> GAMAQQKLDVKWIDKGINWIVYSAKDRENFTMDRWAKFYVNGEIAFCIEPNKEAAIGAVHTGANLDTLFKDQALRNKLTMISHFGYIANKDQSDEQYI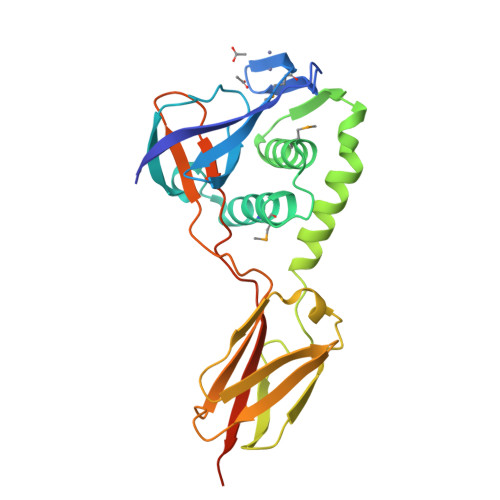ATQMLIWELLGAKYHTIYNGLNYEARKADILKSVKEAEQRASFHKQKKPIKVGEKGVFVDTNNTLSNVKGIRTPSGVNAKIEGNKLIVTADKNAPDNATIHLDRITIVGTPLVYTSGNAQKVGVLKPFDPLDSWLTLQVIKNGNVKIIKEDTETG> PRVKAAQ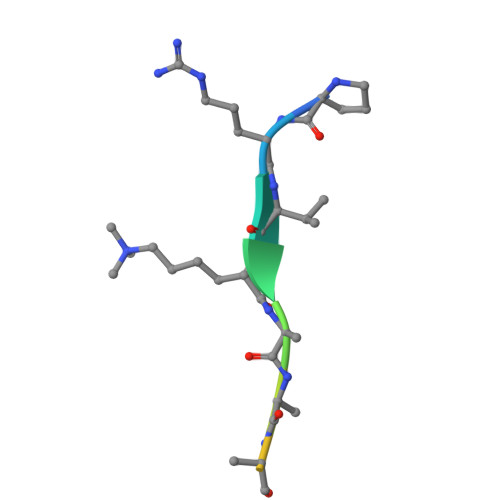AGRQS4-(3,4-dihydro-2H-1,5-benzodioxepin-7-yl)-4-oxobutanoic acid | C13 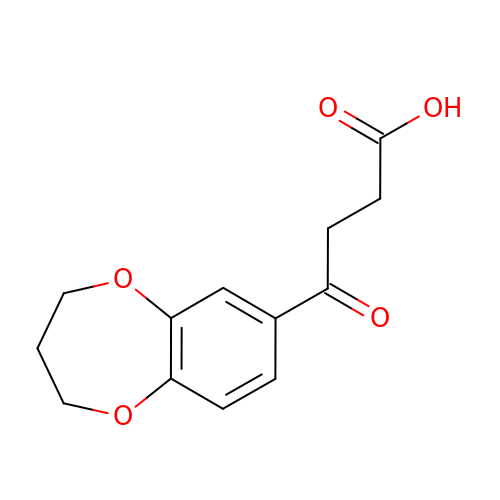H14 O5 | RQYNFIARXFWNDM-UHFFFAOYSA-N4-([1,2,4]triazolo[1,5-a]pyridin-5-yl)benzonitrile | C13 H8 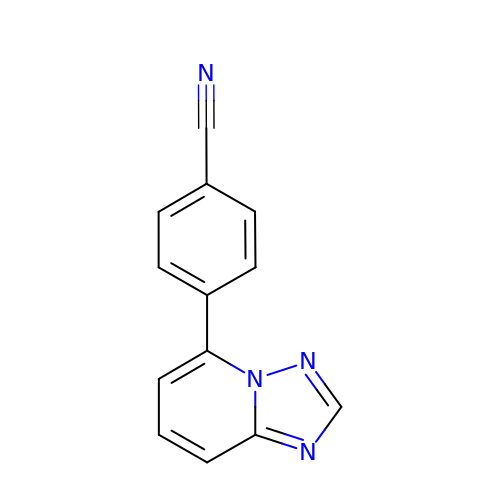N4 | DEYMFBHALUHGST-UHFFFAOYSA-N>MRGSH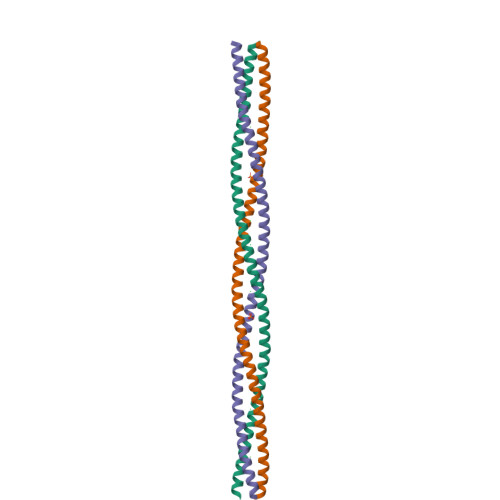HHHHHGSATSANTDRIATAELGIAENKKDAQIAKAQANENKDGIAKNQADIQLHDKKITNLGILHSMVARAVGNNTQGVATNKADIAKNQADIANNIKNIYELAQQQDQHSSDIKTLAKVSAANTDRIAKNKAEADASFETLTKNQKLCSQA[2x]1-(3-acetyl-4,5-dihydroxy-7-methoxynaphthalen-2-yl)propan-2-one 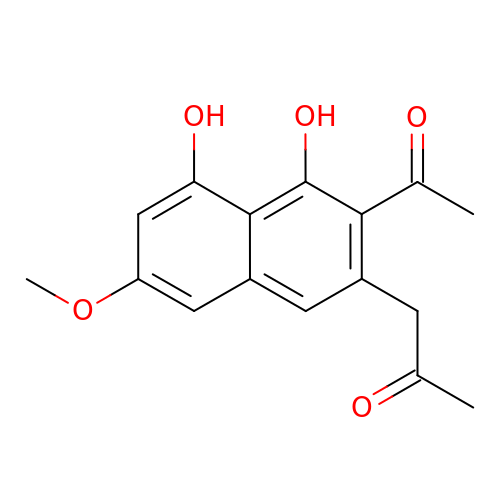| C16 H16 O5 | BONGITCDOWZART-UHFFFAOYSA-N>MVLGKPQTDPTLEWFLSHCHIHKYPSKSTLIHQGEKAETLYYIVKGSVAVLIKDEEGKEMILSYLNQGDFIGELGLFEEGQERSAWVRAKTACEVAEISYKKFRQLIQVNPDILMRLSAQMARRLQVTSEKVGNLAFLDVTGRIAQTLLNLAKQPDAMTHPDGMQIKITRQEIGQIVGCSRETVGRILKMLEDQNLISAH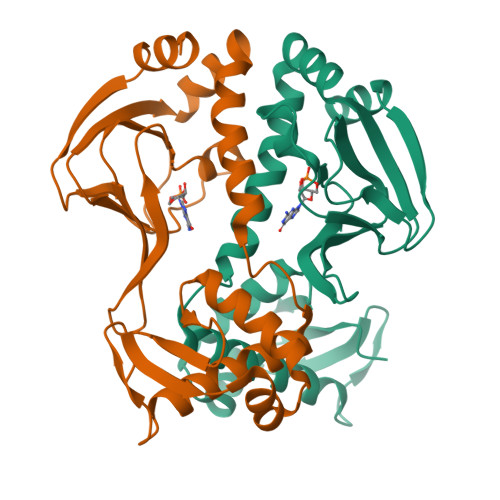GKTIVVYGTR[4x]>GSHMDDALRGELASALDTEGHALPFDVHLQQPHSSGDGTAGDTSTIQLEKLSHPPARFDLLTNSFVYKWQTKAALARKVSGPMREWAAELKYRTGVHIELEPTYPERLSENAVKGSGSDDGDGTQWGAYETADDVDITVYLFGSERGIFNCHKLMEAAIQQDPVYVRLGIFRRLANSSEVEWLMLRRINRELRPPDIPPISLKLPGKWTLLYERYKEAAIRTLWEETGITVDASNVYPTGHLYQTVPQYYWRVPVRYFVAEVPSDIRVEGPQVVPLQYMRNWDARLLRQSPDPIDRAWAQLADPATGCAWMKASMIDQLQKPLRGDNYMAIRYTPPPYSNLQEVVGLGDGSITPSTGNGEDAS[2x]

The 5′ ends are processed by a pyrophosphohydrolase complex termed the PPsome, which is composed of the so-called mitochondrial edited mRNA stability factors 1–3 (MERS1–MERS3). MERS1 was shown to be the factor responsible for catalyzing the 5′ processing event while MERS2 and MERS3 activates its catalysis. Interestingly, the MERS1 Nudix motif (KWTLLYERYKEAAIRTLWEETGI) lacks one of the key metal ion coordinating acidic residues, which in MERS1 is a threonine instead of an acidic residue. The MERS1 structure reveals that it is comprised of two α−β domains.

To address this question and obtain insight into RNA binding by MERS1, we next obtained crystals of MERS1 in complex with an RNA binding site, 5′-GAGAGGGGGGUU-3′, and solved the structure to 2.6 Å resolution. The MERS1–RNA structure contains two MERS1 subunits in the ASU. In the structure, density is evident for four RNA nucleotides bound to each MERS1 subunit. Strikingly, the third nucleotide constructed in the structure, which is the best resolved of the RNA, overlaps the position of the guanine nucleotide in our MERS1–GDP structure. The well-resolved nature of this third guanosine suggests it as the linchpin in RNA binding and supports the notion that the GTP binding site in the MERS1–GTP structure does not represent the location of the bound 5′ nucleotide of its RNA substrate. Of the four bound RNA nucleotides in the MERS1–RNA complex, three have contacts that would provide selectivity for guanine bases and hence they were constructed as guanosines. Comparison of the MERS1–RNA and MERS1–GTP structures revealed that RNA binding induces conformational changes in the RNA binding pocket; Superimposition of the MERS1–GTP and MERS1–RNA structures results in an rmsd of 1.3 Å for corresponding Cα atoms with the significant conformational changes between them found in the RNA binding pocket. Specifically, L2, comprised of residues 222–230, which covers the RNA binding pocket and is unique to MERS1, shifts by ∼3–4 Å to accommodate the RNA. The largest conformational change however occurs within residues 111–128 whereby the helix composed of residues 116–125 shifts as a unit away from the RNA pocket. MERS1 stabilizes its RNA in a single-stranded conformation.>RQLVSNGFEVNLPDQVEVIVRDLPDPSKVKEERTRLMGYWFVHWFDGKLFHLRIKAGGPNVDGEHRAIRTAEHPWLLRARLDDALEEALPKYAAVKKRPFTFLAQKDELIDAAATAAGLSHRLLNSFKVIPRFALSPKIYEPVDGTTRVGVFVTIGMRYDIEASLRDLLEAGIDLRGMYVVRRKRQPGERGLLGRVRAISDDMVQLFEETDLASVNVNDAKLEGSKENFTRCLSALLGHNYKKLLNALDDQEAGYRTGPRFDDAVRRMGEFLAKKPIRLADNINAQVGDRIVFSNEGQARNVRLAPKVEYVFDRTGAKSAEYAWRGLSQFGPFDRPSFANRSPRILVVYPSSTQGKVENFLSAFRDGMGSNYSGFSKGFVDLMGLTKVEFVMCPVEVSSADRNGAHTKYNSAIEDKLAGAGEVHAGIVVLFEDHARLPDDRNPYIHTKSLLLTLGVPTQQVRMPTVLLEPKSLQYTLQNFSIATYAKLNGTPWTVNHDKAINDELVVGMGLAELSGSRTEKRQRFVGITTVFAGDGSYLLGNVSKECEYEGYSDAIRESMTGILRELKKRNNWRPGDTVRVVFHAHRPLKRVDVASIVFECTREIGSDQNIQMAFVTVSHDHPFVLIDRSERGLEAYKGSTARKGVFAPPRGAISRVGRLTRLL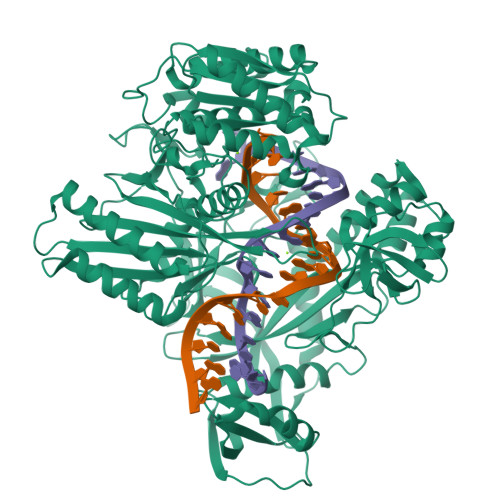AVNSPQLIKRANTPLPTPLLVSLHPDSTFKDVDYLAEQALKFTSLSWRSTLPAATPVTIFYSERIAELLGRLKSIPNWSSANLNIKLKWSRWFL[2x]> NVKAIFLDMDGTILHENNQAST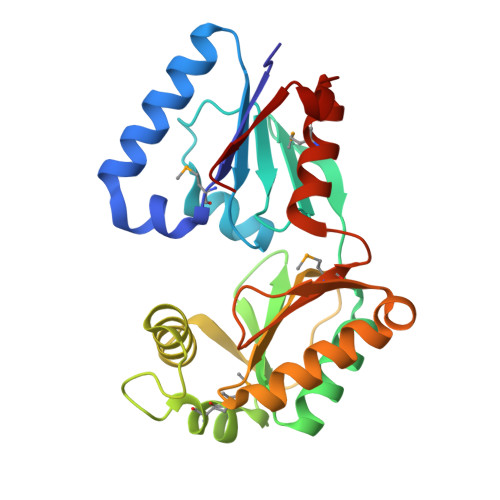YTKDVINQLREKGYKVFLATGRSHSEIHQLVPQDFAVNGIISSNGTIGEVDGEIIFKHGLSLAQVQQITNLAKRQQIYYEVFPFEGNRVSLKEDETWMRDMIRSQDPINGVSHSEWSSRQDALAGKIDWVTKFPEGEYSKIYLFSSNLEKITAFRDELKQNHVQLQISVSNSSRFNAETMAYQTDKGTGIKEMIAHFGIHQEETLVIGD>GSFTEELHLIPPLNFSMVDNGIFRSGFPDSANFSFLQTLGLRSIIYLCPEPYPESNLQFLKSNGIRLFQFGIEGNKEPFVNIPDHKIRMALKVLLDEKNHPVLIHCKRGKHRTGCLVGCLRKLQKWCLTSIFDEYQRFAAAKARVSDQRFMEIFDVSSFSHIPMSFSCSIR[2x]

Here, we provide the ligand/enzyme crystal complexes for one such PTP outlier: Arabidopsis thaliana Plant and Fungi Atypical Dual Specificity Phosphatase 1 (AtPFA-DSP1), herein unveiled as a regioselective and efficient phosphatase towards inositol pyrophosphate (PP-InsP) signaling molecules. Although the WPD loop is missing its canonical tripeptide motif, this structural element contributes to catalysis by assisting PP-InsP delivery into the catalytic pocket, for a choreographed exchange with phosphate reaction product. Subsequently, an intramolecular proton donation by PP-InsP substrate is posited to substitute functionally for the absent aspartate/glutamate general-acid. Additionally, we conclude that the hydrolyzed phosphate remains trapped as an enzyme-product complex, until it can be released in a prisoner exchange with another PP-InsP molecule; the latter process is assisted by the WPD loop.

In experiments in which crystals of wild type AtPFA-DSP149–215 were soaked with reduced concentrations of 5-InsP7 at pH 8.0, we observed a near-planar, triangular-shaped electron density consistent with a metaphosphate; all three of its presumed P–O bonds are an appropriate 1.5 Å in length. There was no evidence of a pentacovalent phosphorane that would have signified an associative reaction pathway. The putative metaphosphate intermediate in wild type enzyme is stabilized by intensive polar contacts with a cluster of residues in the P-loop, Lys151, Arg152, Lys154, His155, and Arg156, including the latter’s positively charged guanidinium group. A metaphosphate is an excellent target for capturing a polarized water molecule, to generate the Pi end-product. We identified a potential candidate, Wat2, in both wild type and Cys150Ser mutant enzymes, and in both cases Wat2 could be activated by the His155 Janus residue. The Nδ1 in His155 is in the Nε2-protonated τ tautomer state, stabilized by a carbonyl oxygen from the backbone of Lys186. In addition, a π-cation interaction can be formed between Arg188 and His155 which is expected to further assist the latter’s deprotonation. Nevertheless, in the wild type enzyme, the 3.7 Å distance and 144° angle from Wat2 to the metaphosphate are not an optimal environment for this reaction, which in addition to the latter’s intensive contacts with P-loop residues (see above), are factors that may assist our crystallographic capture of this proposed intermediate state.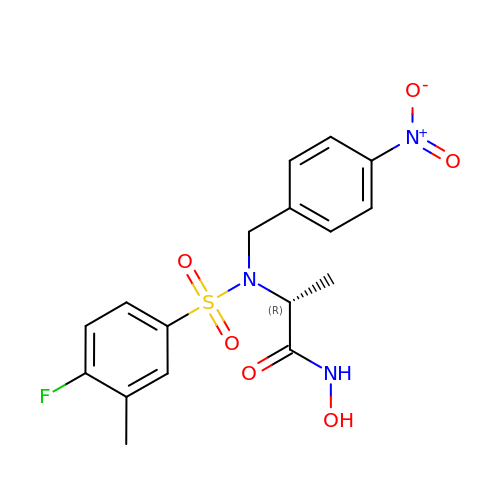N~2~-[(4-fluoro-3-methylphenyl)sulfonyl]-N-hydroxy-N~2~-(4-nitrobenzyl)-D-alaninamide | C17 H18 F N3 O6 S | CUVKDHHEPRADRD-GFCCVEGCSA-N>[4x]GSHMNNEGTKELKLKKLSDNVYQHISYKRVEPWGLIGASGLVVINGTEAHMIDTPWTTQGTKQLIEWIEAKGLTIKSA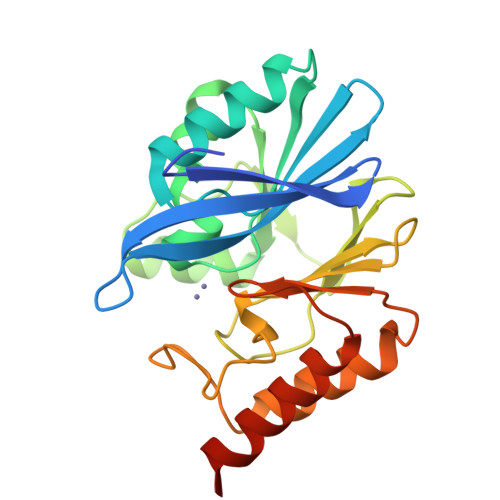VVTHFHEDASGDIPLLNDLKIKTYATSLTNKLLKLNQKEVSSDEISSNTFEFIDGVASVFYPGAGHTEDNIVVWLPNEKILFGGCFVKSLKNKNLGYTGDANISEWPNSMQKVINRYPDAKLVVPGHGEVGDVSLLKHTQALALSAAASNKKINKD> GHMTKLEQ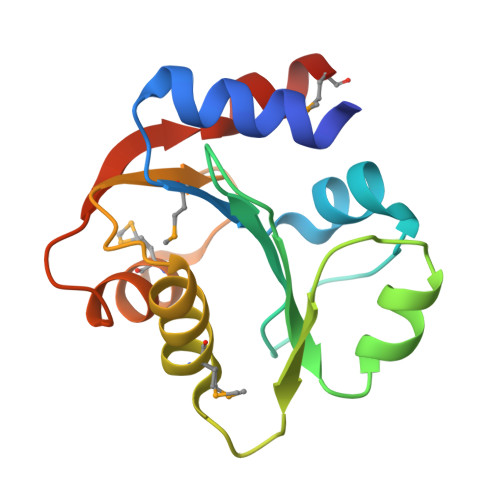IQQWTAQHHASMTYLSNPKTIEYLTGFGSDPIERVLALVVFPDQDPFIFAPALEVEVIKETGWQFPVIGYLDHENPWAMIADQVKQRHVNPEHVAIEKGQLQVARMEALAAQFSAPSFDLDITSFIEHMRGS> HHEGAGTIKQRTLKNIIRATGVGLHSGEKVYLTLKPAPVDTGIVFSRTDLDPVVEIPARAENVGETTMSTTLVKGDVKVDTVEHLLSAMAGLGIDNAYVELSASEVPIMDGSAGPFVFLIQSAGLQEQEAAKKFIRIKREVSVEEGDKRAVFVPFDGFKVSFEIDFDHPVFRGRTQQASVDFSSTSFVKEVSRARTFGFMRDIEYLRSQNLALGGSVENAIVVDENRVL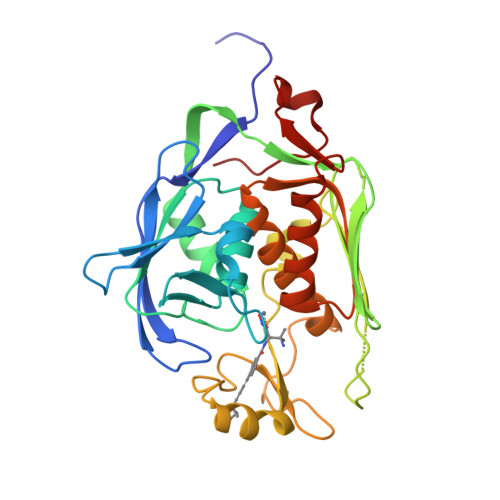NEDGLRYEDEFVKHKILDAIGDLYLLGNSLIGEFRGFKSGHALNNQLLRTLIADKDAWEVVTFEDARTAPISYMRP MSL1, predicted to contain five transmembrane helices and localized to the inner membranes of mitochondria, is involved in the regulation of membrane potential and maintenance of redox homeostasis under abiotic stress. When heterologously expressed in giant E. coli spheroplasts, MSL1 displays stretch-activated gating in excised patches and channel properties similar to those of E. coli MscS (EcMscS), which demonstrates that MSL1 forms a functional mechanosensitive channel. The overall architecture and domain organization of the heptameric AtMSL1 channel resemble those of the EcMscS channel. Akin to TM3 in EcMscS, the innermost helix TM5 is kinked such that TM5a lines the pore and TM5b runs tangentially to the central pore axis and connects to the middle and C-terminal domains, which are located in the mitochondrial matrix.

We expressed an AtMSL1 construct consisting of amino acids 80–497, which lacks the mitochondrial targeting sequence, in the yeast P. pastoris and determined the cryo-EM structure at an overall resolution of ~3.1 Å. Density for the first N-terminal transmembrane helix TM1, which is located at the outer perimeter, is present in the cryo-EM map but rather weak, and thus TM1 is not modeled in the structure. The bowl-shaped transmembrane domain of AtMSL1 suggests that it naturally resides in locally curved, rather than planar, biological membranes. The cryo-EM structure was determined in detergent micelles that are virtually devoid of lipids. The corresponding residues in AtMSL1, V319 and F323, likely play an equivalent role in forming a hydrophobic gate. Pore radius calculation reveals that F323, near the C-terminal end of the pore-lining helix TM5a, defines the narrowest constriction along the central permeation pathway, which is comparable to the closed EcMscS gate in dimension. This indicates that the AtMSL1 structure represents a non-conducting, resting state, which is consistent with the absence of membrane tension in detergent micelles and lipid nanodiscs where the structures were determined. Under low tension, the transmembrane region of AtMSL1 is curved.

>[7x]MSSKSDDFGSIVASGVTGSGDGNGNGNDWVEKAKDVLQTSVDAVTETAKKTKDVSDEMIPHVQQFLDSNPYLKDVIVPVSLTMTGTLFAWVVMPRILRRFHTYAMQSSAKLLPVGFSNEDVPYEKSFWGALEDPARYLVTFIAFAQIAAMVAPTTIAAQYFSPTVKGAVILSLVWFLYRWKTNVITRMLSAKSFGGLDREKVLTLDKVSSVGLFAIGLMASAEACGVAVQSILTVGGVGGVATAFAARDILGNVLSGLSMQFSRPFSMGDTIKAGSVEGQVIEMGLTTTSLLNAEKFPVLVPNSLFSSQVIVNKSRAQWRAIASKIPLQIDDLDMIPQISNEIKEMLRSNTKVFLGKEAPHCYLSRVEKSFAELTIGCNLIRMGKEELYNTQQEVLLEAVKIIKKHGVSLGTTWDNSTLSNSLEVLFQ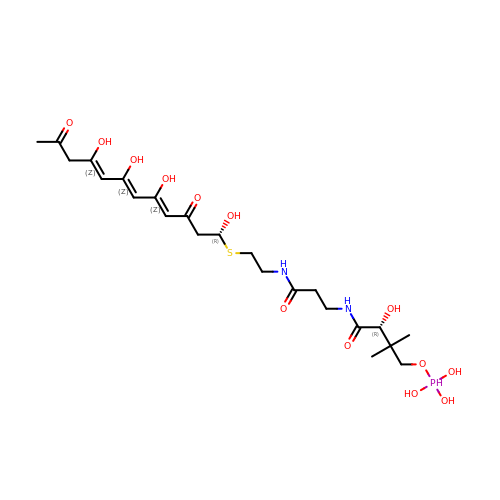(2~{R})-3,3-dimethyl-2-oxidanyl-~{N}-[3-oxidanylidene-3-[2-[(1~{R},4~{Z},6~{Z},8~{Z})-1,5,7,9-tetrakis(oxidanyl)-3,11-bis(oxidanylidene)dodeca-4,6,8-trienyl]sulfanylethylamino]propyl]-4-[tris(oxidanyl)-$l^{5}-phosphanyl]oxy-butanamide | C23 H39 N2 O13 P S | FQZZDEAQTCCCMT-XOXVVNQZSA-N>MAGVETAVRQIELKWPNVPEQLIKGDKFLKWEEGSSSFTEILLRVDPKGYFLYWKIEGKEDSQLLDLAYLRDIRCAKYAKPPKDKKVKDAGTNFGSSNIPLQDKCVTICHGYNYIDLDWIHLVAENSSVAAKWAEEVFSYAYNLLSLNKNQLGEWEKLYFRLTTVEMEKNKIPVKSIQKCLSKDKDDRTRVAKAIEKIGWPSGKNDAIEIKAFDFDTFFKFYLSLLERSEIEGIFKELSQNKGNITTVMFRDFLNDMQRHPSLHKTLFPLYTDSQCDALINEYESAVNKKGKKKGQLTKEGLLYFLMCEENNLTPMHRLDLGANMKLSLAAYYINSSHNTYLTGHQLTGKSSVEIYRQVLLTGCRCLELDCWDGKDGEPIITHGFTMCTEVQFKDVVHAIAECAFKVSEYPVILSFENHCSVPQQKLLAQYCHEAFGELLLDNPIDGHPLKPGVPLPTPYDLRKKILIKNKKIHKGAGDDDELAGLTDEEKKKIEKEKKDAGTAAKEAEAAEEMSALVNYIQPVHFTTFEQAQKKDRHYEMSSMVETQALNKLKDNPEDFVDYNKKQLTRIYPKGTRVDSSNYVPQIYWNAGCQLVALNFQCFDVAMCVNLGVFEYNGCSGYLLKPEFMRKLDKRFDPFTESTVDGVVAGTIEIKIISAQFLSDKQISSYVEVEMYGLPTDTVRKKFKTKTVNNNGMDPYYNENAFVFKKVVLPDLAVVRIIVNEDGGKFIGHRLMPLDGIKPGYRHIPLRNESNRPLGLASVFAHIVAKDYVSDAFAD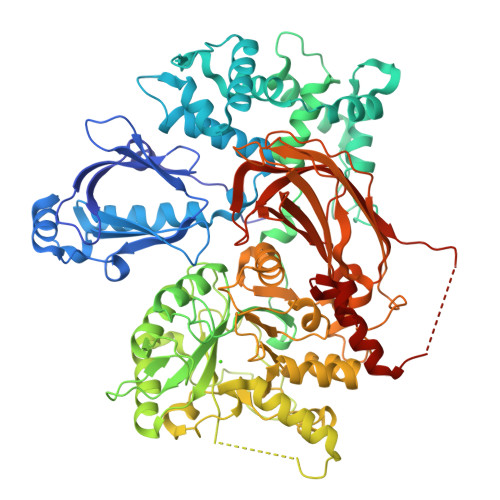FADALLNPIAYQSAQDARAAALCAFEDDPDAALN[2x]11-[(2~{S})-2-[(2-pyridin-3-ylquinazolin-4-yl)amino]-2,3-dihydro-1~{H}-inden-5-yl]undec-10-ynoic acid | C33 H34 N4 O2 | 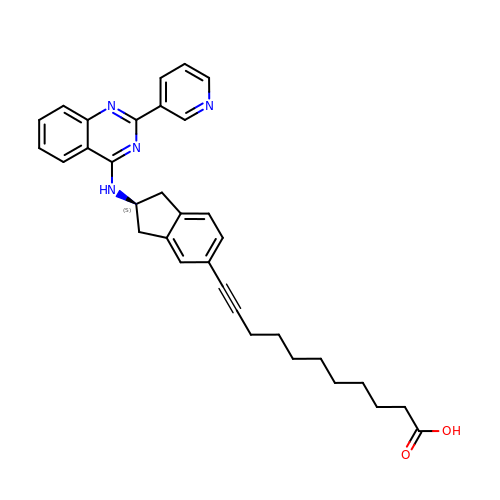OOVVDXXXFLHSBX-NDEPHWFRSA-N>[2x]QQSRNRSTQSQDVARVSSASDYNSSELKTACRKHELYVSFQDLGWQDWIIAPK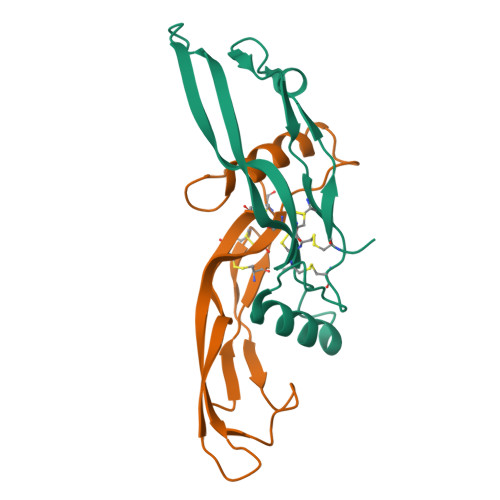GYAANYCDGECSFPLNAHMNATNHAIVQTLVHLMNPEYVPKPCCAPTKLNAISVLYFDDNSNVILKKYRNMVVRACGCH> ANTSSAYNSVYDFLRYHDRGDGLTVNGKTSYSIDQAAAQITRENVSWNGTNVFGKSANLTFKFLQSVSSIPSGDTGFVKFNAEQIEQAKLSLQSWSDVANLTFTEVTGNKSANITFGNYTRDASGNLDYGTQAYAYYPGNYQGAGSSWYNYNQSNIRNPGSEEYGRQTFTHEIGHALGLAHPGEYNAGEGDPSYNDAVYAEDSYQFSILSYWGENETGADYNGHYGGAPMIDDIAAIQRLYGANMTTRTGDSVYGFNSNTDRDFYTATDSSKALIFSVWDAGGTDTFDFSGYSNNQRINLNEGSFSDVGGLKGNVSIAHGVTIENAIGGSGNDILVGNSADNILQGGAGNDVLYGGAGADTLYGGAGRDTFVYGSGQDSTVAAYDWIADFQKGIDKIDLSAFRNEGQLSFVQDQFTGKGQEVMLQWDAANSITNLWLHEAGHSSVDFLVRIVGQAAQSD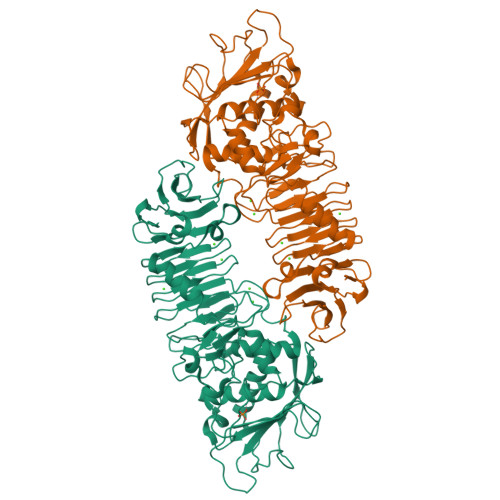IIV>MSVIKSDMKIKLRMEGTVNGHKFVIEGEGEGKPYEGTQTMNLKVKEGAPLPFAYDILTTVFHYGNRVFAKYPKHIPDYFKQSFPEGYSWERSMTFEDGGICTARNDITLEGDCFFNEIRFDGVNFPPNGPVMQKKTLKWEPSTEKMYVRDGVLTGDINMA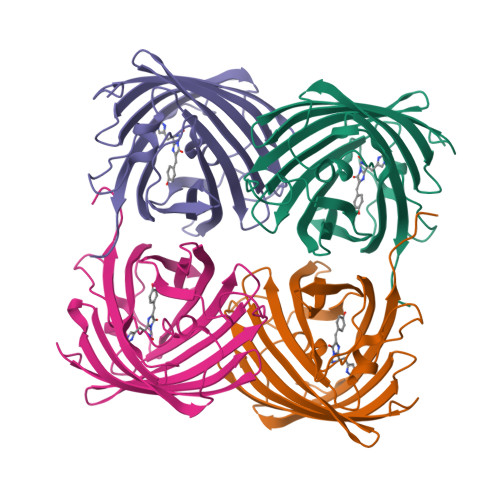LLLEGGGHYRCDFKTTYKAKKGVQLPDYHFVDHCIEILSHDKDYNNVKLYEHAVAHSGLPRQAKHHHHHH[4x]> MEVDIALPTLSPGDLSALQRCEGRVVFLETLRRHATLREVALPCGGDVLAAMAAYRRRFAAVITRVTPHRMLATPLGVGGRGQSLVLQNTGPFDLTNGDHVCLVPPLLGDECLRLTSANLELRFPMTLPLAQARELTARVVARAAETLRGGAPARGADVVFSNGRRYQLPPPHRDNAEAATRSLVLNMIFLLNEGAVILLSLIPNLLT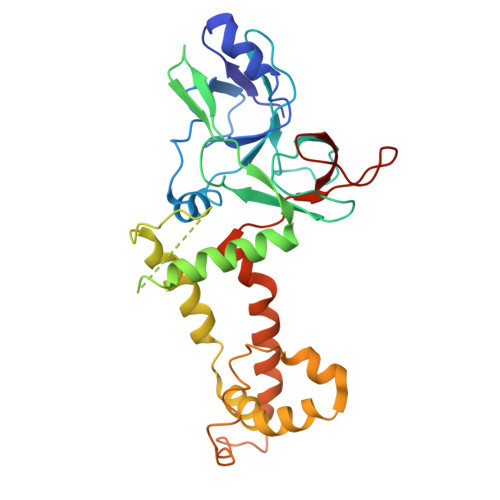LGAQDGYANAVIQLGSATRELGQLVRQPPPPLPQDHARRFCVFEALEAWIASASRLGDTLGTRPVARVCIFDGPPTVPPGEKAAVVEV> SNASKMSDVKCTSVVLLSVLQQLRVESSSKLWAQCVQLHNDILLAKDTTEAFEKMVSLL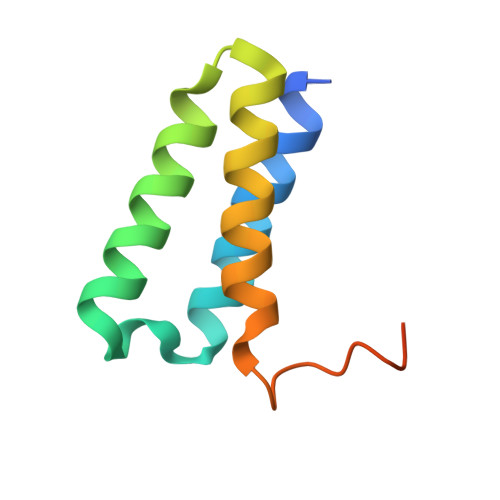SVLLSMQGAVDINKLCEEMLDNRAT>[4x]ILPDSVDWREKGCVTEVKYQGSCGACWAFSAVGALEAQLKLKTGKLVSLSAQNLVDCSTEKYGNKGCNGGFMTTAFQYIIDNKGIDSDASYPYKAMDQKCQYDSK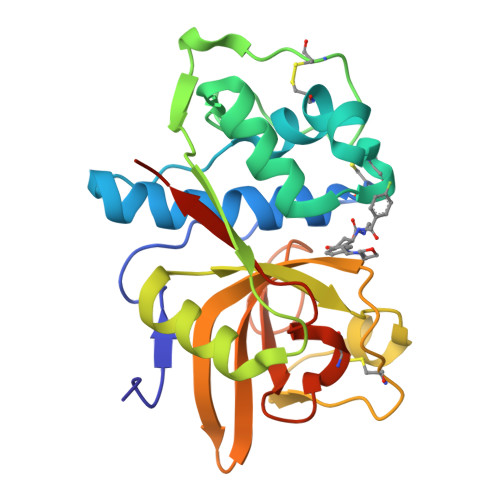YRAATCSKYTELPYGREDVLKEAVANKGPVSVGVDARHPSFFLYRSGVYYEPSCTQNVNHGVLVVGYGDLNGKEYWLVKNSWGHNFGEEGYIRMARNKGNHCGIASFPSYPEIEGHHHHHH>[6x]GSMASHELDYRILGESMQTVEIELDPGETVIAEAGAMNYMTGDIRFTARM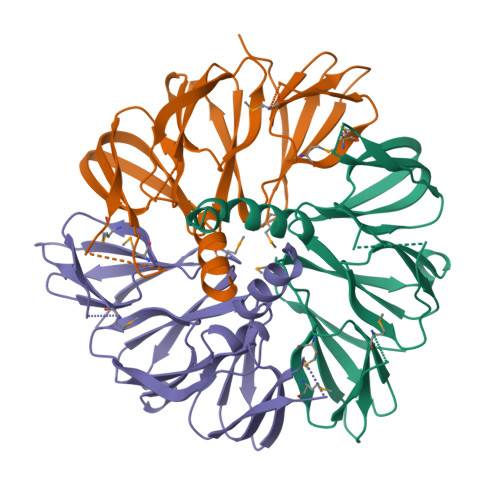GDGSDGSLLGKLWSAGKRKLGGESVFMTHFTNEGQGKQHVAFAAPYPGSVVAVDLDDVGGRLFCQKDSFLCAAYGTRVGIAFTKRLGAGFFGGEGFILQKLEGDGLVFVHAGGTLIRRQLNGETLRVDTGCLVAFTDGIDYDVQLAGGLKSMLFGGEGLLLTTLKGSGTVWLQSLPFSRLAGRIYDATFRAREEVRTNNG>MLTRLKQLQTSTKGYIGIPIVLLMILAMVILPLPPLLLDALFTFNIVLAILVLLVSTTAKRPLDFSVFPTILLVATLLRLTLNVASTRIVLLEGHNGGDAAGKVIQAFGEVVIGGNYVVGMVVFIILMIINFVVITKGGERISEVSARFTLDALPGKQMAIDADLNAGLIDQETARLRRKEVANEADFHGSMDGASKFVRGDAVAGLLILFINIIGGISIGVFEHGLPASEAFKTYALLTIGDGLVAQIPSLLLATAAAIIVTRINDSDNGMSETMQKQLLATPATLFTVAGIMAVIGMVPGMPHLAFFAFAGALGFAGWRQSKKPVQDTQIEQVEALSQAMQEEDTPLTWDDIPHVHTLSLALGYRLVHLVNKDQGAPLSQRIRGVRRNLSEQVGFLLPEVRIRDNLSLKPNQYTISLNGEVIEQGFIEPERLMAIAVGDTYGEIDGILGSDPAYQLPAVWIEHQDKAKALNMGYQVVDDGTVIATHISKIMKTNLAELFTHDDVEAMTQRLTQQAPKLAEALAAALN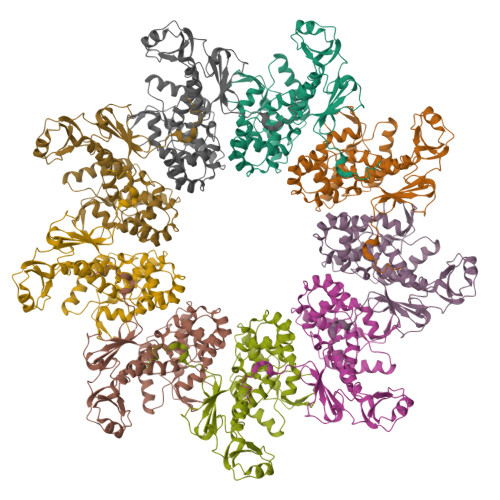PAQQLKVYRQLLLDQVPLKDIRTIANTMLESSENTKDPILLAADVRCALKRTLVNLIAGQKPELNVYALSDELEQMLLTSLQQAQASGTVVLDSFPIEPNILGQFQQNLPLIRQQLKQQGLPPILLVMPQLRPLLARYARTFTQGLAVLSYNEIPENKQINVVGNLGENLYFQ[9x]>MHHHHHHTTTPTVTVLGLGPMGQALSRALLDAGHTVTVWNRTESKAQALRDRGALSAPTPAAAIAASDLALVNVVDHDAVDAILTAAGDAPAGRTVIGLSSDTPDRARRTAKLVGNVGGRYLDGAIMTPIDTIGTRGASILFAGPQALFDEHRGVLDTLGQLTWVGEDHGRAAAFDMALLDLFWTSVGGFGHALMVARANGIEPSELMPHAHGIVGILSPIFTEVAQRVEDDRHSDASASVSSVASSV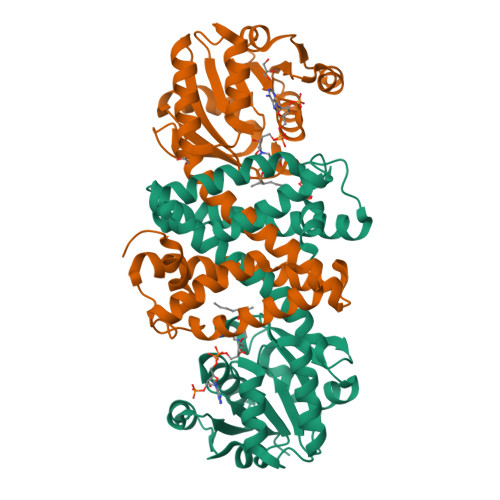RHLIAASREAGVDAGLLEAFRGYVDATVAAGHGDDEISRIASEMTTLTRG[5x]>[8x]MPTKAVTFYEDINYGG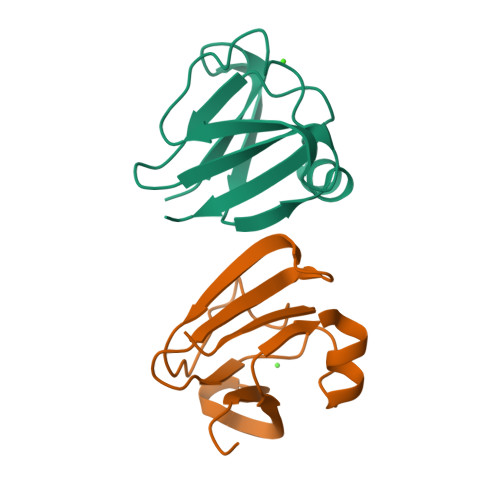ASVSLQPGNYTLSQLNTAKIPNDWMSSLKVPSGWTVDVYENDNFTGTKWTYTSDTPWVGNDANDKMSSVKIYSTTNTGGDT Malyl-CoA lyase (MCL) is a promiscuous carbon-carbon bond lyase that catalyzes the reversible cleavage of structurally related Coenzyme A (CoA) thioesters. Malyl-CoA lyases are promiscuous enzymes that accept a variety of substrates and can catalyze the reversible aldol condensation of CoA thioesters like acetyl-CoA or propionyl-CoA with 2-oxoacids like glyoxylate or pyruvate. The two MCLs share the common fold of a central TIM-barrel with small elaborations, as well as an additional C-terminal domain. In both cases the oligomeric state constitutes a dimer of trimers.

The recombinant MCLR was also initially crystallized in the absence of substrates. The crystals grew in space group P 1 21 1 with one hexamer per AU. Diffraction of the crystals reached a resolution of 2.1 Å and the structure was solved by molecular replacement. Three of the six chains lacked electron density for the entire C-terminal lid domains and were modeled only to Pro265 or Ser266. For the other 3 chains it was possible to model the lid domains with the exception of only the terminal 1, 3, or 8 residues. Notably, of the three lid domains that could be modeled only two were in the closed conformation. Interestingly, in the two subunits where the lid domains were in the closed conformation, the active sites contained electron density that allowed modeling of glyoxylate molecules together with magnesium ions. Nevertheless, Mg2+ could also be fitted into the 4 open active sites, whereas glyoxylate was replaced by water molecules in these subunits. Although glyoxylate was not intentionally present, it was likely carried over from E. coli cell extracts during enzyme purification. Soaking of these crystals with propionyl-CoA resulted in the additional occupancy of one of the two closed active sites with the CoA thioester.

>[6x]MGHHHHHHHHHHSSGHIEGRHMSFRLQPAPPARPNRCQLFGPGSRPALFEKMAASAADVINLDLEDSVAPDDKAQARANIIEAINGLDWGRKYLSVRINGLDTPFWYRDVVDLLEQAGDRLDQIMIPKVGCAADVYAVDALVTAIERAKGRTKPLSFEVIIESAAGIAHVEEIAASSPRLQAMSLGAADFAASMGMQTTGIGGTQENYYMLHDGQKHWSDPWHWAQAAIVAACRTHGILPVDGPFGDFSDDEGFRAQARRSATLGMVGKWAIHPKQVALANEVFTPSETAVTEAREILAAMDAAKARGEGATVYKGRLVDIASIKQAEVIVRQAEMISA4-[2,4-bis(oxidanylidene)-6-(trifluoromethyl)-1H-pyrimidin-3-yl]-5-fluoranyl-2-(2-methylphenoxy)benzenecarbonitrile | C19 H11 F4 N3 O3 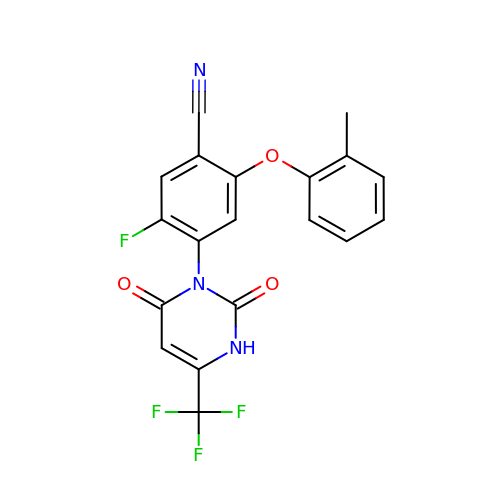| QAJPTKHORNTZSQ-UHFFFAOYSA-N> TPEVGELIEKVRKAHQETFPALCQLGKYTTNNSSEQRVSLDIDLWDKFSELSTKCIIKTVEFAKQLPGFTTLTIADQITLLKAACLDILILRICTRYTPEQDTMTFSDGLTLNRTQMHNAGFGPLTDLVFAFANQLLPLEMDDAETGLLSAICLICGDRQDLEQPDRVDMLQEPLLEALKVYVRKRRPSRPHMFPKMLM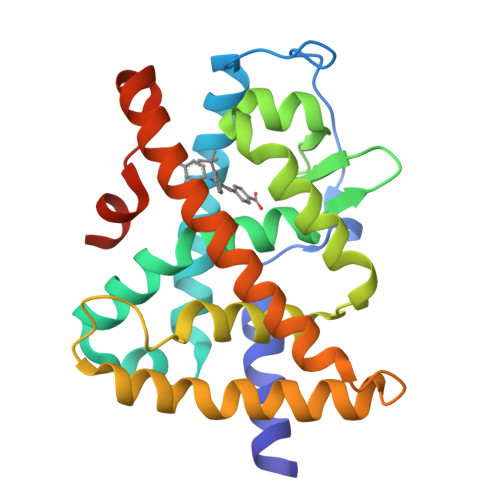KITDLRSISAKGAERVITLKMEIPGSMPPLIQEMLENSEGLDTLSGQ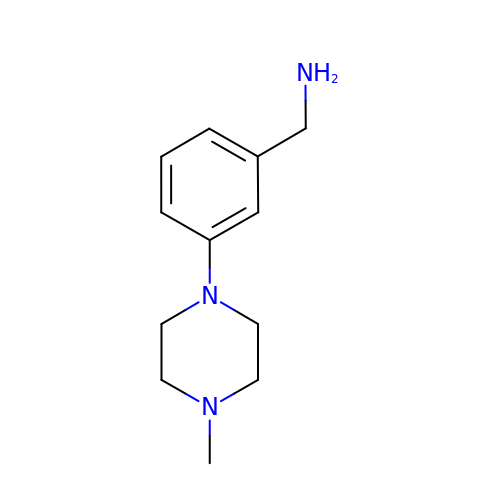1-[3-(4-METHYLPIPERAZIN-1-YL)PHENYL]METHANAMINE | C12 H19 N3 | VKTLTRIKVYJVOX-UHFFFAOYSA-N>[4x]SMASIEIPLHEIIRKLERMNQKKQAQRKRHKLNRKERGHKSPSEQ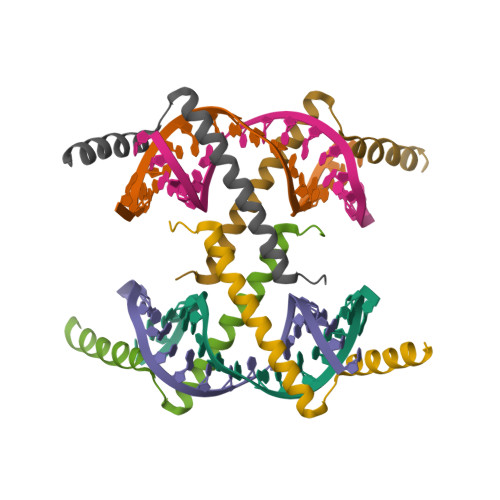RRSELWHARQVELSAINSDNSSDEG>[2x]GPGSMKVEKVFFVTSPIYYVNAAPHIGHVYSTLITDVIGRYHRVKGERVFALTGTDEHGQKVAEAAKQKQVSPYDFTTAVAGEFKKCFEQMDYSIDYFIRTTNEQHKAVVKELWTKLEQKGDIYLGRYEGWYSISDESFLTPQNITDGVDKDGNPCKVSLESGHVVTWVSEENYMFRLSAFRERLLEWYHANPGCIVPEFRRREVIRAVEKGLPDLSVSRARATLHNWAIPVPGNPDHCVYVWLDALTNYLTGSRLRVDESGKEVSLVDDFNELERFPADVHVIGKDILKFHAIYWPAFLLSAGLPLPKKIVAHGWWTKDRKKISKSLGNVFDPVEKAEEF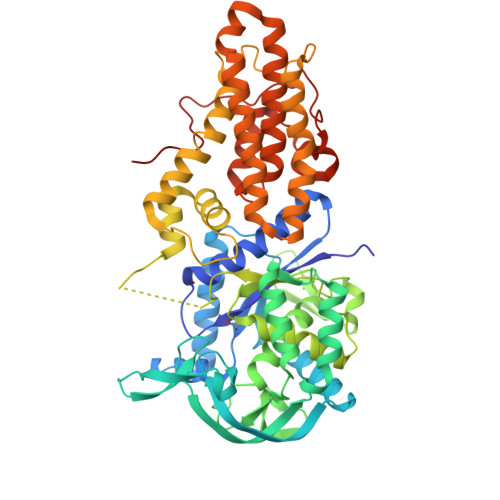GYDALKYFLLRESGFSDDGDYSDKNMIARLNGELADTLGNLVMRCTSAKINVNGEWPSPAAYTEEDESLIQLIKDLPGTADHYYLIPDIQKAIIAVFDVLRAINAYVTDMAPWKLVKTDPERLRTVLYITLEGVRVTTLLLSPILPRKSVVIFDMLGVPEVHRKGIENFEFGAVPPGTRLGPAVEGEVLFSKRSTENTKST> MESVERKSESSYLGMRNMQPEQRLSLDPPRLRSTPQDELHDLLCVGFGPASLAIAIALHDALDPRLNKSASNIHAQPKICFLERQKQFAWHSGMLVPGSKMQISFIKDLATLRDPRSSFTFLNYLHQKGRLIHFTNLSTFL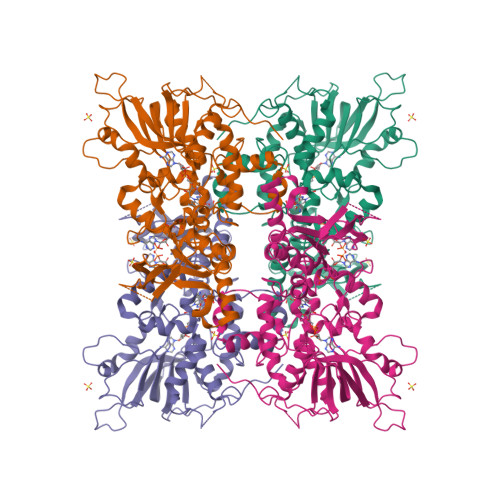PARLEFEDYMRWCAQQFSDVVAYGEEVVEVIPGKSDPSSSVVDFFTVRSRNVETGEISARRTRKVVIAIGGTAKMPSGLPQDPRIIHSSKYCTTLPALLKDKSKPYNIAVLGSGQSAAEIFHDLQKRYPNSRTTLIMRDSAMRPSDDSPFVNEIFNPERVDKFYSQSAAERQRSLLADKATAYSVVRLELIEEIYNDMYLQRVKNPDETQWQHRILPERKITRVEHHGPQSRMRIHLKSSKPESEGAANDVKETLEVDALMVATGYNRNAHERLLSKVQHLRPTGQDQWKPHRDYRVEMDPSKVSSEAGIWLQGCNERTHGLSDSLLSVLAVRGGEMVQSIFGEQLERAAVQGHQLRAML>TVNWEDRPSTPTILGYEVMEERAKFTVYKILVKKTPEESWVVFRRYTDFSRLNDKLKEMFPGFRLALPPKRWFKDNYNADFLEDRQLGLQAFLQNLVAHKDIANCLAVREFLCL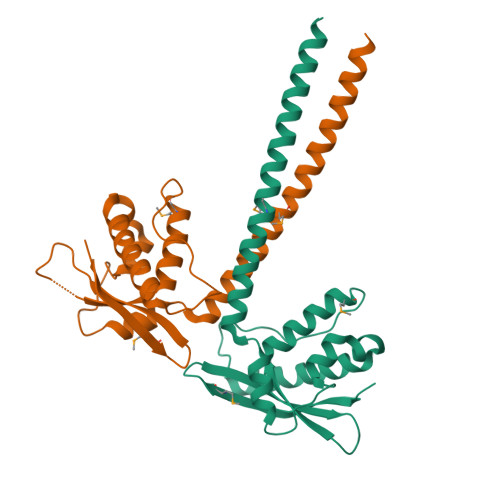DDPPGPFDSLEESRAFCETLEETNYRLQKELLEKQKEMESLKKLLSEKQLHIDTLENRIRTLSLE[6x]>[2x]MIRNIAIIGLGTMGPGMAARLARGGLQVVAYDVAPAAIERARSMLSVAETVLDALGIALPSAGVGTVRFTDDIGDAVSGADLVIENVPENISIKADVYRTIDGLIGQDTI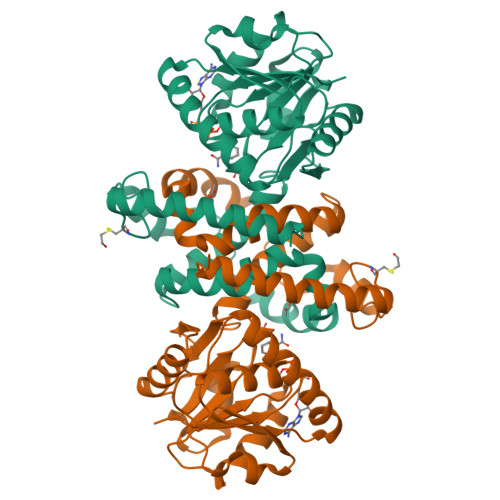VASDTSGIPITKLQAHISYPERMVGMHWSNPPHIIPMIEVIAGEKTAPQTVATIRDLIRSIGLLPVVVKKDVPGFVENRVLYALLREAVDLVERGVIDPEDLDTCVSWGIGYKIAVIGPMALLDMAGLDIYKSVSSFLNADLSNRDDVAPMVLEKTSASKFGIKSGEGMFCYTPEQTKALQAERARKLVAVRRILEGRE>[2x]MGAAILPDLGTEILIPVCAVIGIAFALFQWLLVSKVKLSAVRDASPNAAAKNGYNDYLIEEEEGINDHNVVVKCAEIQNAISEGATSFLFTEYKYVGIFMVAFAILIFLFLGSVEGFSTSPQACSYDKTKTCKPALATAIFSTVSFLLGGVTSLVSGFLGMKIATYANARTTLEARKGVGKAFITAFRSGAVMGFLLAANGLLVLYIAINLFKIYYGDDWGGLFHAITGYGLGGSSMALFGRVGGGIYTKAADVGADLVGKVERNIPEDDPRNPAVIADNVGDNVGDIAGMGSDLFGSYAESSCAALVVASISSFGLNHELTAMLYPLIVSSVGILVCLLTTLFATDFFEIKAVKEIEPALKKQLVISTVLMTIGVAVVSFVALPTSFTIFNFGVQKDVKSWQLFLCVAVGLWAGLIIGFVTEYYTSNAYSPVQDVADSCRTGAATNVIFGLALGYKSVIIP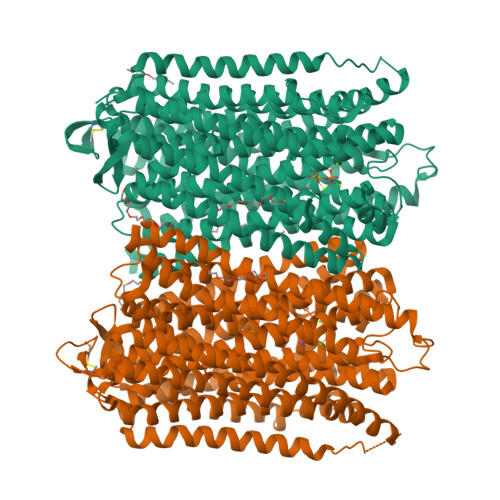IFAIAISIFVSFTFAAMYGIAVAALGMLSTIATGLAIDAYGPISDNAGGIAEMAGMSHRIRERTDALDAAGNTTAAIGKGFAIGSAALVSLALFGAFVSRASITTVDVLTPKVFIGLIVGAMLPYWFSAMTMKSVGSAALKMVEEVRRQFNTIPGLMEGTAKPDYATCVKISTDASIKEMIPPGALVMLTPLVVGILFGVETLSGVLAGSLVSGVQIAISASNTGGAWDNAKKYIEAGASEHARSLGPKGSDCHKAAVIGDTIGDPLKDTSGPSLNILIKLMAVESLVFAPFFATHGGLLFKIF> IVGGYTCGANTVPYQVSLNSGYHFCGGSLINSQWVVSAAHCYKSGIQVRLGEDNINVVEGNEQFISASKSIVHPSYNSNTLNNDIMLIKLKSAASLNSRVASISLPTSCASAGTQCLISGWGNTKSSGTSYPDVLKCLKAPILSDSSCKSAYPGQITSNMFCAGYLEGGKDSCQGDSGGPVVCSGKL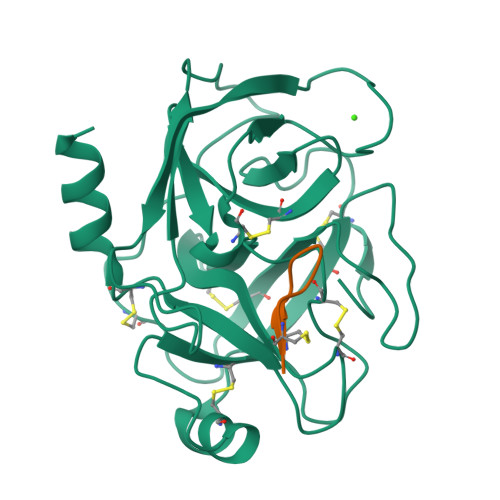QGIVSWGSGCAQKNKPGVYTKVCNYVSWIKQTIASN;> SCTRSIPPQCY> ACGTCT;> GAACGACAAAGACGTCGAGTC;> TCGAGTCG;> T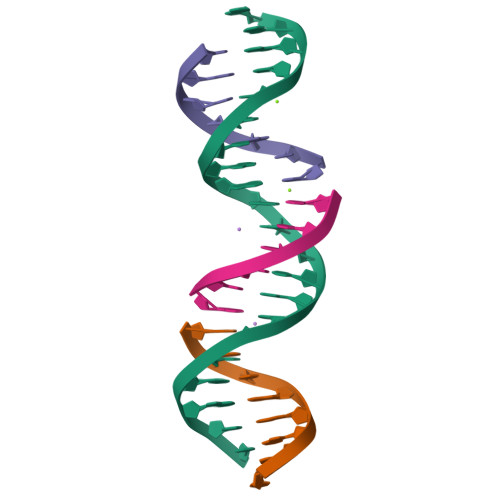TGTCGT benzyl [(2S)-1-(3-nitrophenyl)-3-oxobutan-2-yl]carbamate | C18 H18 N2 O5 | 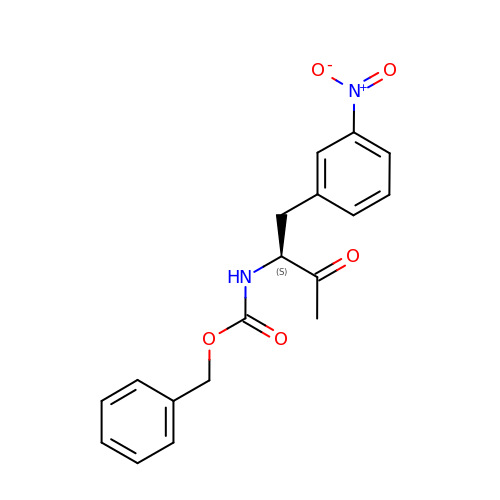XMNMBBOQTUQLRM-KRWDZBQOSA-N> MGQSKKLNKQPSSLSPLVQLAGIRKCFDGKEVIPQLDLTIN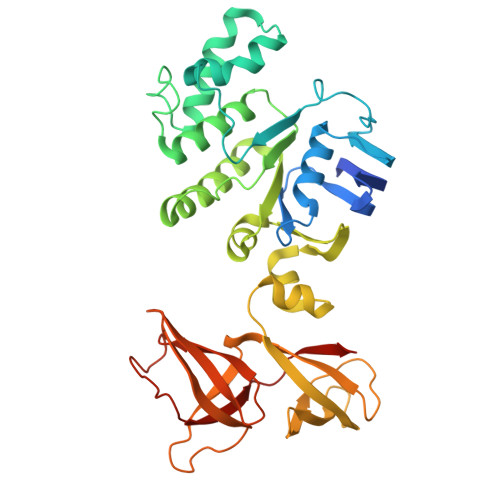NGEFLTLLGPSGCGKTTVLRLIAGLETVDSGRIMLDNEDITHVPAENRYVNTVFQSYALFPHMTVFENVAFGLRMQKTPAAEITPRVMEALRMVQLETFAQRKPHQLSGGQQQRVAIARAVVNKPRLLLLDESLSALDYKLRKQMQNELKALQRKLGITFVFVTHDQEEALTMSDRIVVMRDGRIEQDGTPREIYEEPKNLFVAGFIGEINMFNATVIERLDEQRVRANVEGRECNIYVNFAVEPGQKLHVLLRPEDLRVEEINDDNHAEGLIGYVRERNYKGMTLESVVELENGKMVMVSEFFNEDDPDFDHSLDQKMAINWVESWEVVLADEEHK> MATPLAVNSAASLWGPYKDIWHKVGNALWRRQPEAVHLLDKILKKHKPDFISLFKNPPKNVQQHEKVQKASTEGVAIQGQQGTRLLPEQLIKEAFILSDLFDIGELAAVELLLAGEHQQPHFPGLTRGLVAVLLYWDGKRCIANSLKALIQSRRGKTWTLELSPELASMTTRFTDELMEQGLTYKVLTLVSQIDVNNEFEKLQRERGLGSEKHRKEVSDLIKECRQSLAESLFAWACQSPLGKEDTLLLIGHLERVTVEANGSLDAVNLALLMALLYCFDISFIEQSTEERDDMIHQLPLLTEKQYIATIHSRLQDSQLWKLPGLQATVRLAWALALRGISQLPDVTALAEFTEADEAMAELAIADNVFLFLMESVVVSEYFYQEEFYIRRVHNLITDFLALMPMKVKQLRNRADEDARMIHMSMQMGNEPPISLRRDLEHLMLLIGELYKKNPFHLELALEYWCPTEPLQTPTIMGSYLGVAHQRPPQRQVVLSKFVRQMGDLLPPTIYIPYLKMLQGLANGPQCAHYCFSLLKVNGSSHVENIQGAGGSPVSWEHFFHSLMLYHEHLRKDLPSADSVQYRHLPSRGITQKEQDGLIAFLQLTSTIITWSENARLALCEHPQWTPVVVILGLLQCSIPPVLKAELLKTLAAFGKSPEIAASLWQSLEYTQILQTVRIPSQRQAIGIEVELNEIESRCEEYPLTRAFCQLISTLVESSFPSNLGAGLRPPGFDPYLQFLRDSVFLRFRTRAYRRAAEKWEVAEVVLEVFYKLLRDYEPQLEDFVDQFVELQGEEIIAYKPPGFSLMYHLLNESPMLELALSLLEEGVKQLDTYAPFPGKKHLEKAVQHCLALLNLTLQKENLFMDLLRESQLALIVCPLEQLLQGINPRTKKADNVVNIARYLYHGNTNPELAFESAKILCCISCNSNIQIKLVGDFTHDQSISQKLMAGFVECLDCEDAEEFVRLEEGSELEKKLVAIRHETRIHILNLLITSLECNPPNLALYLLGFELKKPVSTTNLQDPGVLGCPRTCLHAILNILEKGTEGRTGPVAVRESPQ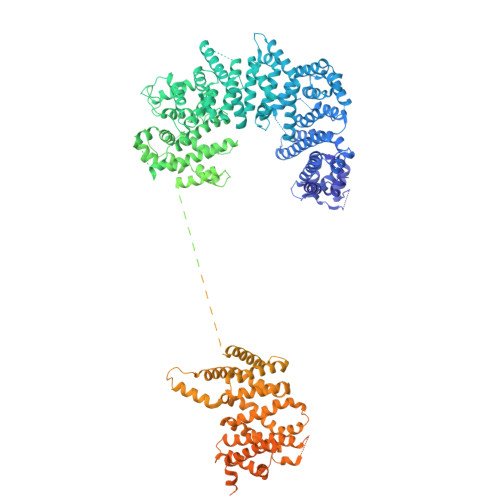LAELCYQVIYQLCACSDTSGPTMRYLRTSQDFLFSQLQYLPFSNKEYEISMLNQMSWLMKTASIELRVTSLNRQRSHTQRLLHLLLDDMPVKPYSDGEGGIEDENRSVSGFLHFDTATKVRRKILNILDSIDFSQEIPEPLQLDFFDRAQIEQVIANCEHKNLRGQTVCNVKLLHRVLVAEVNALQGMAAIGQRPLLMEEISTVLQYVVGRNKLLQCLHAKRHALESWRQLVEIILTACPQDLIQAEDRQLIIRDILQDVHDKILDDEAAQELMPVVAGAVFTLTAHLSQAVLTEQKETSVLGPAEAHYAFMLDSCFTSPPPEENPLVGFASIGDSSLYIILKKLLDFILKTGGGFQRVRTHLYGSLLYYLQIAQRPDEPDTLEAAKKTMWERLTAPEDVFSKLQRENIAIIESYGAALMEVVCRDACDGHEIGRMLALALLDRIVSVDKQQQWLLYLSNSGYLKVLVDSLVEDDRTLQSLLTPQPPLLKALYTYESKMAFLTRVAKIQQGALELLRSGVIVRLAQCQVYDMRPETDPQSMFGMRDPPMFIPTPVDRYRQILLPALQLCQVILTSSMAQHLQAAGQVLQFLISHSDTIQAILRCQDVSAGSLQELALLTGIISKAALPGILSELDVDVNEGSLMELQGHIGRFQRQCLGLLSRFGGSDRLRQFKFQDDNVEGDKVSKKDEIELAMQQICANVMEYCQSLMLQSSPTFQHAVCLFTPSLSETVNRDGPRQDTQAPVVPYWRLPGLGIIIYLLKQSANDFFSYYDSHRQSVSKLQNVEQLPPDEIKELCQSVMPAGVDKISTAQKYVLARRRLVKVINNRAKLLSLCSFIIETCLFILWRHLEYYLLHCMPTDSQDSLFASRTLFKSRRLQDSFASETNLDFRSGLAIVSQHDLDQLQADAINAFGESLQKKLLDIEGLYSKVRSRYSFIQALVRRIRGLLRISRN4-methyl-~{N}-undecyl-pyridine-1-carboxamide | C18 H36 N2 O | 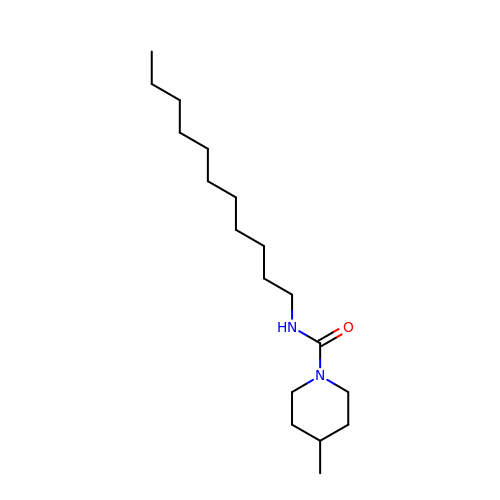SYMUTLCUVXEJOU-UHFFFAOYSA-O> MPSQSGMNPADLSGLSGKELARARRAALSKQGKAAVSNKTASVNRSTKQAASSINTNQVRSSVNEVPTDYQMADQLCSTIDHADFGTESNRVRDLCRQRREALSTIGKKAAKTTGKPSGRVRPQQSVVHNDAMIENAGDTNQSSSTSLNNELSEICSIADDMPERFGSQAKTVRDICRARRQALSERGTRAVPPKPQSQGGPGRNGYQIDGYLDTALHGRDAAKRHREMLCQYGRGTAPSCKPTGRVKNSVQSGNAAPKKVETGHTLSGGSVTGTQVDRKSHVTGNEPGTCRAVTGTEYVGTEQFTSFCNTSPKPNATKVNVTTTARGRPVSGTEVSRTEKVTGNESGVCRNVTGTEYMSNEAHFSLCGTAAKPSQADKVMFGATARTHQVVSGSDEFRPSSVTGNESGAKRTITGSQYADEGLARLTINGAPAKVARTHTFAGSDVTGTEIGRSTRVTGDESGSCRSISGTEYLSNEQFQSFCDTKPQRSPFKVGQDRTNKGQSVTGNLVDRSELVTGNEPGSCSRVTGSQYGQSKICGGGVGKVRSMRTLRGTSVSGQQLDHAPKMSGDERGGCMPV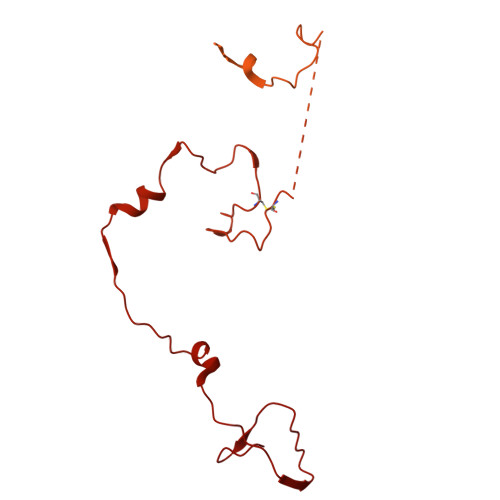TGNEYYGREHFEPFCTSTPEPEAQSTEQSLTCEGQIISGTSVDASDLVTGNEIGEQQLISGDAYVGAQQTGCLPTSPRFNQTGNVQSMGFKNTNQPEQNFAPGEVMPTDFSIQTPARSAQNRITGNDIAPSGRITGPGMLATGLITGTPEFRHAARELVGSPQPMAMAMANRNKAAQAPVVQPEVVATQEKPELVCAPRSDQMDRVSGEGKERCHITGDDWSVNKHITGTAGQWASGRNPSMRGNARVVETSAFANRNVPKPEKPGSKITGSSGNDTQGSLITYSGGARG> APATGG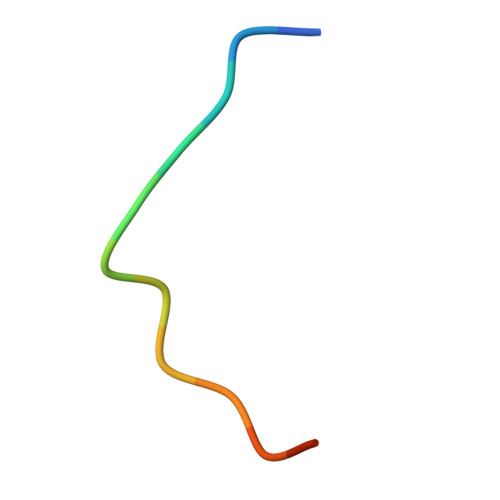VCKPHRY> NNQ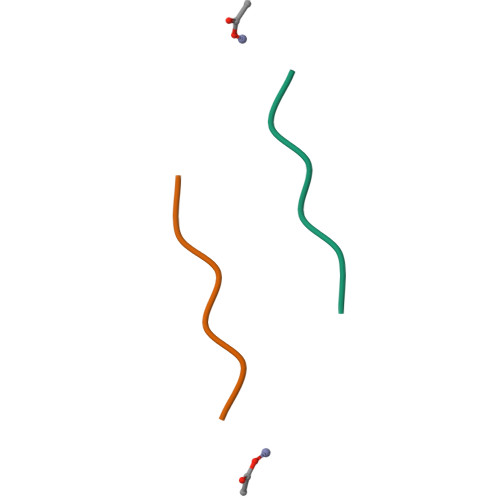QNY> QEARTGNDIAQLPAISVTGREISDLTEGTNAYTTEAMSTATGLTLSPRETPQSVSVVTRQQIEDQGLTDTGAILATAPGISVTRSDSNRYSFSARGFTIDNFQFDGLVSPILSQWNYGSTDMDAAIYDHVEIVRGATGLMTGSGNPSAAVNFVRKRPLREFAATFNASVGSWDYVRGDADISVPITEDGRIRSRLVAAYSQGDSYVHFLDTRRRTFYGVVSADLTPDTVLTTSVEYQHNHSNGFGSGFPLFYSDGSRTDFNRSVANNAPWARQDTEATTYFVDLTHRFTNDWKLRAAYSHTDGRYLMKHVYRGGYPDRHTGIIAAPPAFSNYDGNLDRDDIHFSLSAPFEAFGLRHEVALGWMSIDNHSDIQRYAMVGPAPAIGSFFDWRRAGSHHHHHHHIQEPSWADTLSPADDVRTKQTGAYLVGRFALAEPLHLIVGDRWSDWKTKQMYFGSRREYRIKNQFTPYAGLTYDINDTYTAYASYTEIFQPQNARDTSGGILPPIKSKSYELGLKAAYLEGRLNTSAALFQTRQDNLAQVIPGSSIP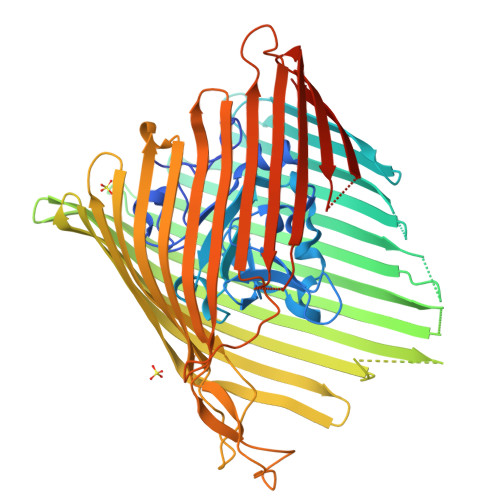GFPNMQASRAASGAKVEGIDLEASGQILPDWNIGASYTHFTTKDASGNPINTNHPRSLFKLYTTYRLPGALHRLTVGGGVDWQSRMYQAAASPRGNVEVEQDSYALVSLMARFDFNKKLSATLNVNNLFDKKYYDQIGFYSQGWWGAPRNVMLNLRAQY> MTEKLKLTKRLVEEYRRFYQVELSKKPSTHAILLPLSKALEQILSVPDDWDEEELILQGSGQLQAALDRQEVYTRPIIKDKSVAYETRQLQELEAIQIFMTTCVRDLFGEMCKGDR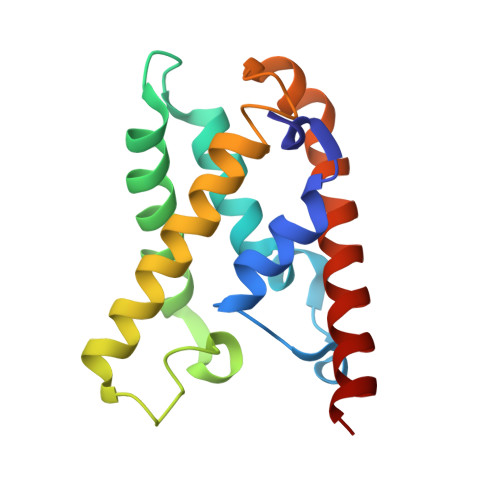AILQEQRNRIKSGAEFAYRLLALEAQQNQN4-[3-[2-chloranyl-6-(trifluoromethyl)phenoxy]-5-(dimethylcarbamoyl)indazol-1-yl]benzoic acid | C24 H17 Cl F3 N3 O4 | 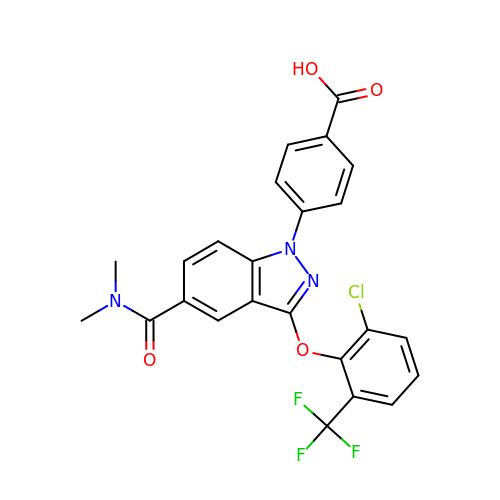PRFOAGMHUSKCKE-UHFFFAOYSA-N> MDALSNGIKKHRTSLPSPMFSRNDFSIWSILRKCIGMELSKITMPVIFNEPLSFLQRLTEYMEHTYLIHKASSLSDPVERMQCVAAFAVSAVASQWERTGKPFNPLLGETYELVRDDLGFRLISEQVSHHPPISAFHAEGLNNDFIFHGSIYPKLKFWGKSVEAEPKGTITLELLEHNEAYTWTNPTCCVHNIIVGKLWIEQYGNVEIINHKTGDKCVLNFKPCGLFGKELHKVEGYIQDKSKKKLCALYGKWTECLYSVDPATFDAYKKNDKKNTEEKKNSKQMSTSEELDEMPVPDSESVFIIPGSVLLWRIAPRPPNSAQMYNFTSFAMVLNEVDKDMESVIPKTDCRLRPDIRAMENGEIDQASEEKKRLEEKQRAARKNRSKSEEDWKTRWFHQGPNPYNGAQDWIYSGSYWDRNYFNLPDIYLEHHHHHH

Members of the OSBP/ORP family vary in length: the short ORPs contain primarily a conserved OSBP-related domain (ORD) that can bind and transfer lipids such as sterols, PIPs or phosphatidylserine (PS), whereas the long ones often possess additional functional domains for ligand binding and/or membrane targeting. The OSBPL1A gene (homo sapiens) encodes two proteins: the long isoform ORP1L (residues 1–950) containing the ANK (ankyrin repeat) domain, the PH (Pleckstrin homology) domain, the FFAT (diphenylalanine in an acidic tract) motif and the ORD, and a short isoform ORP1S (residues 514–950) containing only the ORD. Here, while we cannot rule out its cholesterol sensor function, our structural, biochemical and cell biological data suggest that ORP1L is a bona fide cholesterol transporter. Here, our results suggest that ORP1 is a unique sensor of lysosomal PI-bisphosphates, and that PI(4,5)P2/PI(3,4)P2 allosterically regulates cholesterol transport by ORP1.

To further illustrate the mechanisms underlying cholesterol transport by ORP1-ORD, we solved two crystal structures of ORP1-ORD (524–950 or 534–950) in complex with cholesterol. The most striking feature is that their N-terminal loops (residues 514–546) and lid regions (547–565) adopt different open conformations, distinct from the closed conformations observed in yeast Osh structures. To accomplish the lipid transport function, the ORP/Osh proteins were expected to adopt the open state when extracting lipids from or unloading them onto the membrane, and the closed state when transporting lipids between two membranes. Therefore, the open conformations of ORP1-ORD may represent certain important states when ORP1 exerts physiological functions (see below). In the 3.4 Å structure, the sterol molecule is similarly accommodated in the hydrophobic tunnel. Consistently, structural analyses of the open cholesterol-bound ORP1-ORD revealed domain swapping between symmetry-related molecules, effectively generating dimers or trimers. In these ORP1-ORD oligomers, the N-terminal loop of one molecule is nestled in a shallow groove on the core of a symmetry-related molecule, forming multiple hydrophobic and polar interactions. Thus, the lids in three oligomerization states of the cholesterol-bound ORP1-ORD, though adopting different conformations, can seal the lipid-binding tunnel.> AVLGKEAMLKMQTSNVLILGLKGLGVEIAKNVVLAGVKSMTVFDPEPVQLADLSTQFFLTEKDIGQKRGDVTRAKLAELNAYVPVNVLDSLDDVTQLSQFQVVVATDTVSLEDKVKINEFCHSSGIRFISSETRGLFGNTFVDLGDEFTVLDPTGEEPRTGMVSDIEPDGTVTMLDDNRHGLEDGNFVRFSEVEGLDKLNDGTLFKVE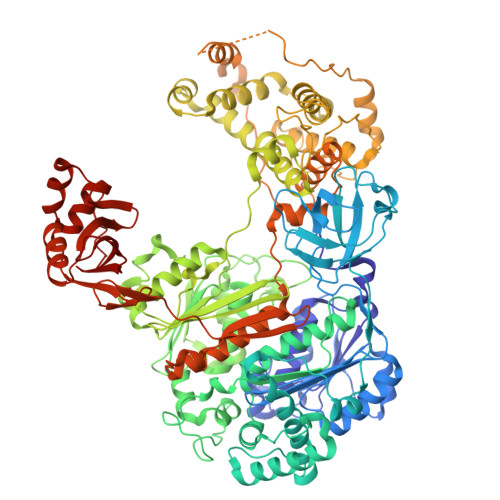VLGPFAFRIGSVKEYGEYKKGGIFTEVKVPRKISFKSLKQQLSNPEFVFSDFAKFDRAAQLHLGFQALHQFAVRHNGELPRTMNDEDANELIKLVTDLSVQQPEVLGEGVDVNEDLIKELSYQARGDIPGVVAFFGGLVAQEVLKACSGKFTPLKQFMYFDSLESLPDPKNFPRNEKTTQPVNSRYDNQIAVFGLDFQKKIANSKVFLVGSGAIGCEMLKNWALLGLGSGSDGYIVVTDNDSIEKSNANRQFLFRPKDVGKNKSEVAAEAVCAMNPDLKGKINAKIDKVGPETEEIFNDSFWESLDFVTNALDNVDARTYVDRRCVFYRKPLLESGTLGTKGNTQVIIPRLTESYSSSRDPPEKSIPLCTLRSFPNKIDHTIAWAKSLFQGYFTDSAENVNMYLTQPNFVEQTLKQSGDVKGVLESISDSLSSKPHNFEDCIKWARLEFEKKFNHDIKQLLFNFPKDAKTSNGEPFWSGAKRAPTPLEFDIYNNDHFHFVVAGASLRAYNYGIKSDDSNSKPNVDEYKSVIDHMIIPEFTPNANLKIQVNDDDPDPNANAANGSDEIDQLVSSLPDPSTLAGFKLEPVDFEKDDDTNHHIEFITACSNCRAQNYFIETADRQKTKFIAGRIIPAIATTTSLVTGLVNLELYKLIDNKTDIEQYKNGFVNLALPFFGFSEPIASPKGEYNNKKYDKIWDRFDIKGDIKLSDLIEHFEKDEGLEITMLSYGVSLLYASFFPPKKLKERLNLPITQLVKLVTKKDIPAHVSTMILEICADDKEGEDVEVPFITIHL>TDTTPPTITLPQEVIAYRGEEFEFFVETTDDSGRVNRVIVRNIEGADNSTYLDPNWIRYSTDNLSVPGNATPANPLRTRVYGIVPINHGVGPGDRYTKYVRAEDAAGNITALVDKQSERFVLVIRPQTEKYTPQVPTLTYVQNANSLTQTDKDAVIAAVKSANPNLPATSTYSVSENGTVTITYPDGSTDTIAAAQTVDTDRVAPVFVDEGRDYIFYRGEEGTAELHFYDNSGKITNVNFAGDLAASSTYNTLLGLGFTFNTPNINNPNNATEQNPLVTTIRGTIPKSLPAGPGGKYTFKVRATDASGLTSEAKIFRIVFANQTDKYTPNNPGSLTGVLNPQQLSTSEKTAIEEKVRAANTGNLPNNVQYVVNNDGSVTVIYPDDTPASRSRDTITADRTVQDLRPR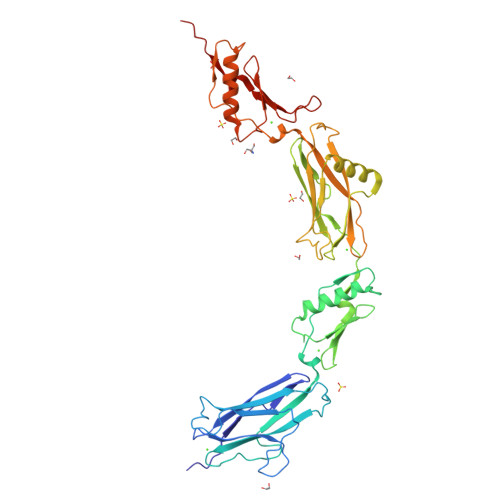NS[2x]> IVGGKDCPKGECPWQVLLLVNGAQLCGGTLINTIWVVSAAHCFDKIKNWRNLIAVLGEHDLSEHDGDEQSRRVAQVIIPSTYVPGTTNHD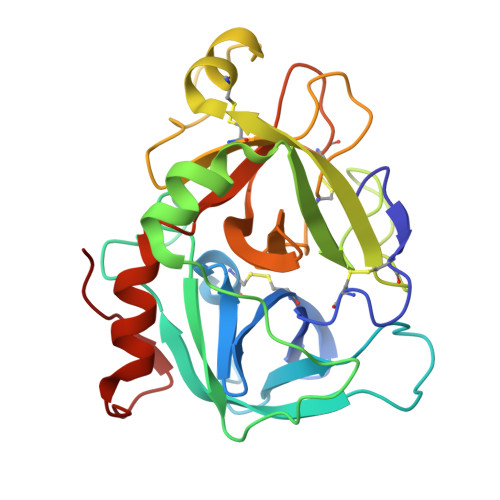IALLRLHQPVVLTDHVVPLCLPERTFSERTLAFVRFSLVSGWGQLLDRGATALVLQVLNVPRLMTQDCLQQSRKVGDSPNITEYMFCAGYSDGSKDSCKGDSGGPHATHYRGTWYLTGIVSWGQGCATVGHFGVYTRVSQYIEWLQKLMRSEPRPGVLLRAPFP TGFBI-related corneal dystrophy (CD) is characterized by the accumulation of insoluble protein deposits in the corneal tissues, eventually leading to progressive corneal opacity. Mutations in the TGFBI gene results in the mutant protein product, TGFBI protein (TGFBIp) which is proteolytically cleaved in the corneal tissues. From our previous proteomics analysis and spatial high-resolution mass spectrometry imaging, we concluded that the TGFBIp is the main component of the amyloid aggregates found in patients’cornea and the TGFBIp-derived peptides are the predominant component of the TGFBIp fibril found in the amyloid deposits, respectively. Since the mechanism of amyloid disassembly by ATP-independent chaperones is unknown, we reconstructed atomic models of the amyloids self-assembled from TGFBIp-derived peptides and their complex with L-PGDS using cryo-EM and NMR.

Biophysical study of different mutants of the 611-633 region of the TGFBIp has revealed that the G623R mutant showed the highest amyloid aggregation propensity and fibril stability. Since this 611-633 region with the G623R mutation of the TGFBIp showed the most microscopically homogeneous fibrils and well-resolved ssNMR spectra, we have chosen it as our primary model system for structural studies. We used a hybrid structure determination approach combining ssNMR and cryo-EM to produce the atomic resolution model of the fibril. Next, we obtained an electron density map of the fibrils with 4.9 Å resolution after 3D refinement. Finally, we obtained the atomic model of the G623R fibrils through the combination of the data obtained from both techniques. From the analysis of the G623R fibril model, the R623 residue is involved in the formation of intermolecular salt-bridge with D617 and E615 in the opposite strand. Furthermore, when we simultaneously swapped the residues participating in this salt bridge in the double mutant (R623D, D617R), uniform fibrils could again be produced, thus validating the presence of this salt bridge in the amyloid model. Additionally, this thermodynamically favorable interaction provided by the inter-strand salt bridge likely accelerates the fibril growth of the G623R peptide compared to wild-type and other mutants. We identified the structurally frustrated interactions within the G623R fibril using the online server, Frustratometer40. From Fig. S13a, b the highly frustrated regions within the G623R fibrils, represented by red lines, are clustered around the β-turn region of the fibril. The β-turn region is enriched with negatively charged residues (E615 and D617) stacked upon each other which experiences strong charge-charge repulsion.

>EPVAEPDIMATNRVVHVITNVLQ[20x]UPF0201 family proteins constitute one such uncharacterized, archaeal specific protein family. The UPF0201 family proteins occur as a single globular α/β domain with approximate dimensions of 55×35×35 Å3. The protomeric structure consists of a five-stranded, anti-parallel β-sheet, five α helices, which are located on one face of the β-sheet, and three loops connecting helices and strands. We have further documented that all members of this archaeal specific protein family share a common polypeptide chain fold, which is evolutionarily related to the RRM motif found in the ribosomal L5 proteins and many other RNA-binding proteins.

For 10077a from M. jannaschii, full-length constructs with either N- or C-terminal His6 affinity tags failed to yield crystals. C-terminal truncation of 30 amino acids yielded diffraction quality crystals and a structure. The polypeptide chains of 10077a and 10077b extend beyond the C-terminal helix, α5, for about 20 residues, and form a type IV turn followed by random coil. Pairwise sequence identities among the structures we report herein range between 15–22%, with exception of 10077a and 10077b, which are 35% identical. Our four UPF0201 structures represent subfamilies N149845 (10077a, b) and N130963 (10077c, d). The crystallographic asymmetric units contain one protomer in 10077c, two in 10077b and four protomers in both 10077a and 10077d. While 10077a, 10077b and 10077d all form one type of dimer (typeI), 10077c forms altogether different dimer via crystallographic symmetry (typeII). The interface surface area for type I dimers in 10077a, 10077b and 10077d are 672, 563 and 611 Å2, respectively. In type I the turn connecting β1 and helix α2 (residues Thr13-Asp15) assemble closely to form a two stranded β-sheet. Interestingly, structure alignment shows residues (Thr13, Glu14, Asp15, and Lys18 of 10077a) near the interface of type I assembly are strictly conserved while those seen at the type II assembly are not.

>SLEVIIKAKVKPTEDKYKVKKAILNIFPKAKLTFIEKDNEFGEWEGKTKSVEKLKELLRSQSILDAARMVLEKGMTENATKFYLNKQAAYVGAVNFDIDTHGGIFVKILADENEDIMKIIKDIAPRTKGGVIINEDELEEGHHHHHH[4x]> GPLGSDHSLNIVTVTLNMERHHFLGISIVGQSNDRGDGGIYIGSIMKGGAVAADGRIEPGDMLLQVNDVNFENMSNDDA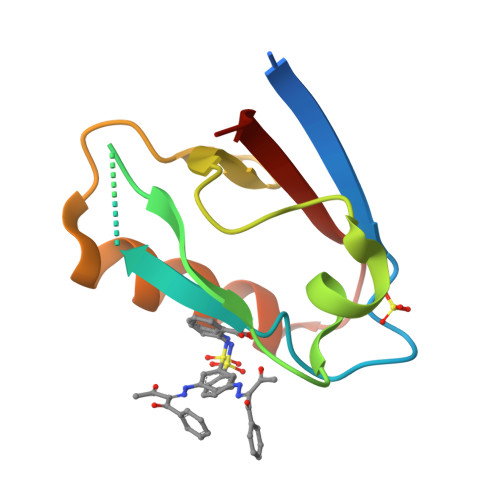VRVLREIVSQTGPISLTVAKATD N~2~-(benzylsulfonyl)-D-arginyl-N-(4-carbamimidoylbenzyl)glycinamide 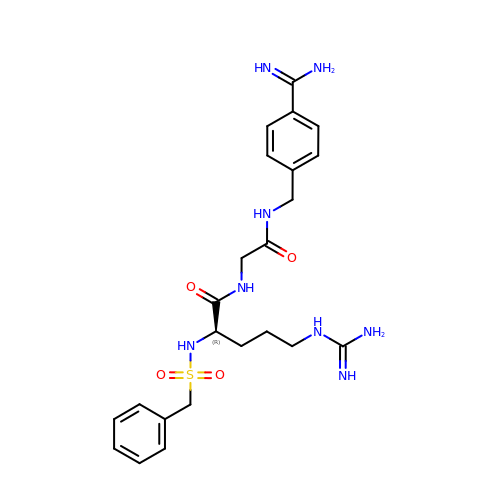| C23 H32 N8 O4 S | MVMUALCRWZYTQR-LJQANCHMSA-N>LGSSNDNIELVDFQNIMFYGDAEVGDNQQPFTFILDTGSANLWVPSVKCTTAGCLTKHLYDSSKSRTYEKDGTKVEMNYVSGTVSGFFSKDLVTVGNLSLPYKFIEVIDTNGFEPTYTASTFDGILGLGWKDLSIGSVDPIVVELKNQNKIENALFTFYLPVHDKHTGFLTIGGIEERFYEGPLTYEKLNHDLYWQITLDAHVGNIMLEKANCIVDSGTSAITVPTDFLNKMLQNLDVIKVPFLPFYVTLCNNSKLPTFEFTSENGKYTLEPEYYLQHIEDVGPGLCMLNIIGLDFPVPTFILGDPFMRKYFTVF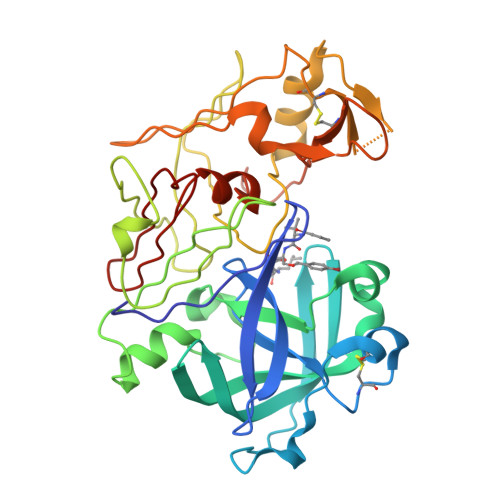DYDNHSVGIALAKKNL[2x]>SVEEIRLPRAGGPLGLSIVGGSDHSSHPFGVQEPGVFISKVLPRGLAARSGLRVGDRILAVNGQDVRDATHQEAVSALLRPCLELSLLVRRD[2x]

The Scribble (Scrib) protein is a conserved cell polarity regulator with anti-tumorigenic properties. Scribble is an important regulator of cell polarity and acts as a scaffolding protein to mediate a diverse set of cellular signalling pathways via its four PDZ domains. The zoonotic Tick-born encephalitis virus TBEV encodes for the NS5 protein, which has been shown to interact with Scribble in a PDZ domain dependent manner. In summary, we show that TBEV NS5 C-terminal PBM binds SCRIB PDZ3 in order to interact with Scribble.

To understand the interactions of SCRIB PDZ domain interactions with NS5 PBM sequences in more detail we determined crystal structures of SCRIB PDZ3:NS5_CTN complexes as well as a structure of SCRIB PDZ3 apo. Binding of NS5_CTN in a non-canonical manner requires no significant change in the SCRIB PDZ3 domain fold, with a superimposition of both SCRIB PDZ3 chains yielding an RMSD of 1.15 Å in Chain A and 1.35 Å in Chain B over the Cα backbone atoms. Furthermore, all side chain rotamers of residues involved in the canonical ligand binding groove are identical with those found in PDZ3:NS5_CTN, including His1071PDZ3. No major changes in B-factor distribution for backbone atoms are observed upon NS5_CTN binding.UGGT acts as the gatekeeper in this system because this enzyme is capable of sensing the folding states of glycoproteins as potential substrates. UGGT only transfers monoglucose residues to incompletely folded glycoproteins. UGGT is a large enzyme, comprising approximately 1500 amino acid residues, which has been putatively divided into two regions: an N-terminal folding-sensor region, which accounts for approximately 80% of the enzyme and is not homologous with any known structures, and a C-terminal catalytic domain, which accounts for the remaining 20% of the enzyme and belongs to the glycosyltransferase 8 family. On the other hand, the folding-sensor region of UGGT was found to harbour three tandem Trx-like domains: Trx1 (residues 168–379), Trx2 (residues 467–624) and Trx3 (residues 671–831).

The final model of Form 1, refined to a resolution of 3.40 Å, had an Rwork of 23.5% and Rfree of 29.2%. The crystal belonged to space group I23 with six molecules per asymmetric unit. The structures of molecules A–F were highly similar to each other with an RMSD value of 0.11–0.37 Å for superimposed Cα atoms 94–155. Molecule A in the crystal structure, which had the lowest average B value, was used for the comparative analysis and will be primarily described hereafter. As expected from the bioinformatics analysis, the crystal structure displayed a typical Trx-like fold, i.e. a five-stranded β-sheet with a β1–β3–β2–β4–β5 arrangement surrounded by six α-helices. In the crystal structure, a part of β5–α6 loop (residues 816–818) was disordered. The C-terminal α6-containing segment showed a higher crystallographic B-factor (87.7 Å2) than the average value (79.7 Å2). The α6 helix was stabilized mainly through its hydrophobic surface, containing Phe820, Phe825, Phe828 and Leu829, which made contact with the hydrophobic patch, including Leu703 (β2), Leu717, Phe724 (α2), Val804, Leu806 (β4), Leu811 (β5) and Ile814 (β5–α6 loop) (right). The Trx3 domain possesses an extensive hydrophobic patch, which is covered by the flexible C-terminal helix and can participate in interactions with hydrophobic molecules. Moreover, we provided snapshots of the 3D structure of the third Trx-like domain, in which a putative substrate-binding hydrophobic patch is intramolecularly masked or involved in an intermolecular interaction, offering a key breakthrough toward understanding of the functional mechanisms of this ER folding-sensor enzyme.

>GSNVNKIYIENHDLMSKVPVIEASKESTRDDWAALTVVADLDDIEGQELVYYALRFRKSNDGVRLDIVHNPKDTSRSPSVLAQRLKSREDKLLDFTRFLDLETALETGEFEPDVAYDASLANFLASSNMKAGDNFVILNGRVLGPITSADDFKKEDFEVFLQA[6x]>[4x]MTKIALIGSGQIGAIVGELCLLENLGDLILYDVVPGIPQGKALDLKHFSTILGVNRNILGTNQIEDIKDADIIVITAGVQRKEGMTREDLIGVNGKIMKSVAESV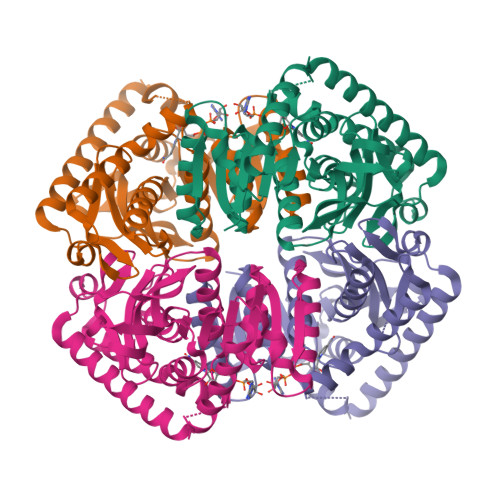KLHCSKAFVICVSNPLDIMVNVFHKFSNLPHEKICGMAGILDTSRYCSLIADKLKVSAEDVNAVILGGHGDLMVPLQRYTSVNGVPLSEFVKKNMISQNEIQEIIQKTRNMGAEIIKLAKASAAFAPAAAITKMIKSYLYNENNLFTCAVYLNGHYNCSNLFVGSTAKINNKGAHPVEFPLTKEEQDLYTESIASVQSNTQKAFDLIKAAALEHHHHHH>GSMAASFFSDFGLMWYLEELKKEEFRKFKEHLKQMTLQLELKQIPWTEVKKASREELANLLIKHYEEQQAWNITLRIFQKMDRKDLCMKV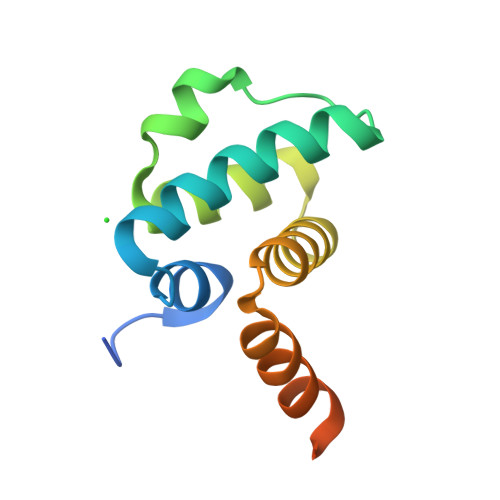MRERTGYTKTYQAHAKQKFSRLE[2x]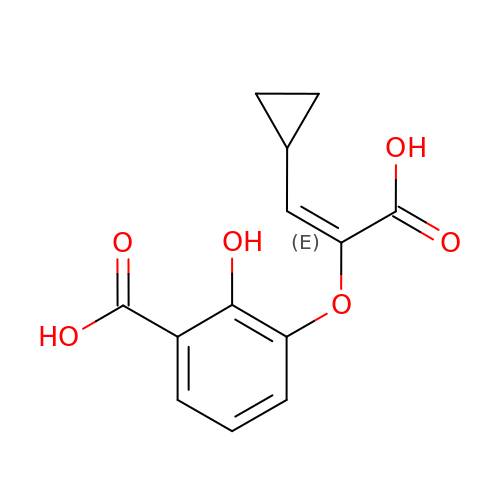3-{[(E)-1-carboxy-2-cyclopropylethenyl]oxy}-2-hydroxybenzoic acid | C13 H12 O6 | RBBOJHGNWUPRCK-UXBLZVDNSA-N>HHHHHHMHTSTTSTVPLEPWTAQQLQQATQGYWHKDQIPQTEIKRILTDSRHAESGDAFLALKGERFDAHNFVAQVVANGCQVAIVERPIDAEIAQLVVADTRLALGQLGAYRREQNAQLKVIALTGSSGKTTTKEMLGSILSRLAPTLITRGNLNNDLGVPMMLLELRKEHQYAVMELGANHQGEIDYTSKIVQPHVAGILNIGTAHLGEFGGRDGICRAKSEIYRHILPQGVAIVPQQDDFTAEIREAAKSHQIMSFGEGGDVFATEIELLPQSANFQLHTPQGSSFVRLPFAGEHNVQNATAAVAFALALGVSLEDIVKGLEQAQGAKGRLNFIQKAPHLFIDDTYNANPTSMRAAAQVLLQQNGIKVMVMGDIGELGDSSWQEHHDLGRDLAELPLDHIVAVGQFASAALEGAGLH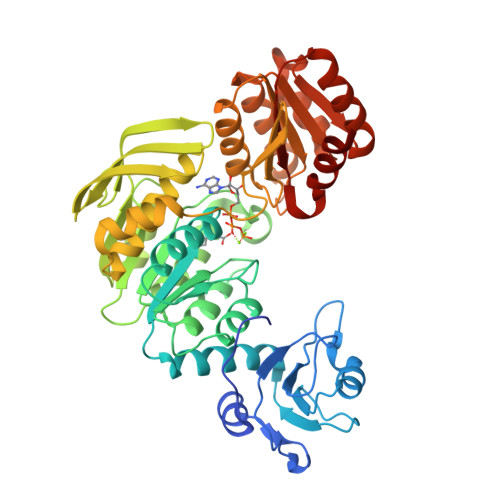STKLKAFQTQAEALPFLINLIQTHQPQSMSFLFKGSRFTHMETLMADLMEKL[2x]>[2x]GMAQGLIEVERKFAPGPDTEERLQELGATLEHRVTFRDTYYDTSELSLMLSDHWLRQREGSGWELKCPGVTGVSGPHNEYVEVTSEAAIVAQLFELLGSGEQKPAGVAAVLGSLKLQEVASFITTRSSWKLALSGAHGQEPQLTIDLDSADFGYAVGEVEAMVHEKAEVPAALEKIITVSSMLGVPAQEEAPAKLMVYLQRFRPLDYQRLLEAASSGEATGDSASS

The Vtc4p β-tunnel domain is not unique to eukaryotic polyP polymerases but is a structural hallmark of triphosphate tunnel metalloenzymes (TTMs), whose characteristic features are the presence of a topologically closed hydrophilic β-barrel, the preference for triphosphate-containing substrates, and for a divalent metal co-factor (PFAM families CYTH and VTC). Members of the ancient triphosphate tunnel metalloenzyme family can be found in all kingdoms of life. Our comparative analysis defines that most of these enzymes share a common catalytic mechanism in their tunnel centers, yet they have evolved different substrate recognition modes on their tunnel entries. The observed substrate plasticity apparently allows TTM proteins to act on a wide array of enzyme substrates and to perform very different reactions, many of which likely remain to be discovered.

We thus structurally characterized a mammalian TTM ThTPase, which was previously shown to specifically hydrolyze thiamine triphosphate (ThTP) into ThDP and Pi. We synthesized ThTP from ThDP and produced co-crystal structures of mouse ThTPase with its substrate at pH 6, where ThTPase catalytic activity is minimal. Consequently, we found an intact ThTP molecule bound in the tunnel center of ThTPase. The thiamine portion of the substrate binds to a pocket generated by the tunnel walls and the C-terminal plug helix, with the thiazole ring making a stacking interaction with Trp-53 and with Met-195 from the plug helix. The ThTP triphosphate moiety binds in the same conformation as outlined for the PPPi-bound structures of AtTTM3 and ygiF above. Our substrate-bound mouse ThTPase structure supports an earlier docking model of human ThTPase. The observed substrate binding mode in mouse ThTPase reinforces the notion that to bind their substrates, TTMs require opening of their closed tunnel domains into a cup-shaped hand, as previously shown by NMR spectroscopy. The unique modes of substrate binding in ThTPases and adenylate cyclases allow these enzymes to carry out rather different reactions and to produce different leaving groups (ortho- and pyrophosphate, respectively) while maintaining a unified cleavage site in close proximity of metal binding site 2. Both the N- and C-terminal sides of the tunnel domain have evolved to recognize specific substrates, as exemplified by our ThTPase structure and by the class IV adenylate cyclase complexes.> GPLGSMNRVEAARNVHIVGSGDTTVVLGHGFGTDQSVWKHLVPYLVDSYRVLLYDNMGAGSTNPEYFHFERYSTLQGYAHDLLVILHEFNIRSCIFVGHSLSAMTGAIASIIRPDLFQKIVMLSASPRFLNTADYLGGFEPADVEQLAGAIEANYKSWVSGFAPMVVGGDMDSVAVQEFSRTLFNMRPDIARSVFRTIFTSDLRDYLGRVTVPCHIIQSSRDMAVPVSVAGYIHNRVGGRSVVEVMNTEGHLPQLSAPEVAIPVLLRHIKNDIDS

Here we present the crystal structure of S. hermonthica intermediate KAI2 (ShKAI2iB), which has 98% sequence identity with ShKAI2i that has been reported to respond to karrikin but not to GR24 through complementation experiments. ShKAI2iB consisted of a core domain and a cap domain. A cavity was formed between the two domains, in common with other KAI2/D14 proteins reported12202122232425, and catalytic triad (Ser95-His246-Asp217) lied at the bottom of the cavity. Our results indicated a novel binding specificity in which ShKAI2iB bound karrikin but not SL, in agreement with the reported results of cross-species complementation assays of ShKAI2i.

To determine why ShKAI2iB exhibited a different binding specificity from KAI2 and D14s, we solved crystal structures of apo ShKAI2iB at 2.0-Å resolution and ShKAI2iB-KAR1 complex at 1.2-Å resolution. In the complex structure of ShKAI2iB-KAR1, KAR1 was embedded completely in the cavity, with the oxygen-bearing edge facing down, and thus, the carbonyl group of KAR1 pointing toward the bottom of the cavity. Carbonyl oxygen of KAR1 in the ShKAI2iB-KAR1 structure was able to form hydrogen bond with the hydroxyl group of Ser95 through a water molecule. This water molecule also formed hydrogen bonds with main-chain amide nitrogen atoms of Phe26 and Leu96, which acts as an oxyanion hole in catalytic activity of α/β hydrolase. On the other hand, the methyl group of KAR1 was embedded in the hydrophobic side consisting of Phe26, Leu142, Phe190, Ile193 and Phe194, and the pyran ring of KAR1 formed face-to-edge aromatic-dipole interactions and hydrophobic interactions with ShKAI2iB. Upon KAR1 binding, Phe194 moved 1 Å away from KAR1 binding site, creating a space to accommodate KAR1. Actually, S95A exhibited almost no heat change following the addition of KAR1 in the ITC experiment, indicating that Ser95 is vital for KAR1 binding, likely by stabilizing a water molecule in the vicinity. As a result of inward shift of helix αD1, the side chain of Leu142 will cause a steric clash with KAR1 if it takes the same orientation as that in the KAI2-KAR1 structure. Unexpectedly, the complexed structure of ShKAI2iB with KAR1 also has a closed cavity, indicating that conformational changes of the cap domain are required to enable KAR1 to access the cavity. In the structure of KAR1-bound ShKAI2iB, the cavity was closed and KAR1 was unable to be exposed to the solvent.>[2x]GS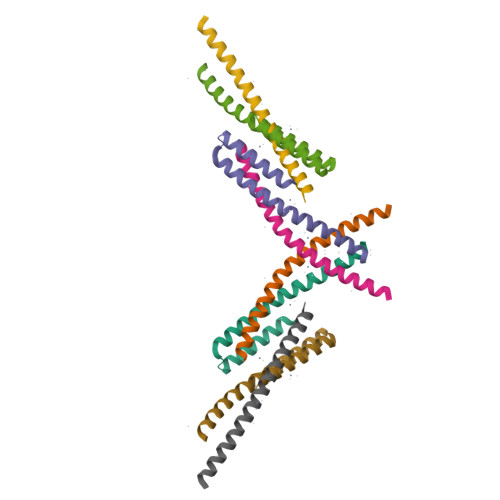SLENLPPVAASIEQLLERQWSEGQQFLLEQGTPSDILGMLKSLHQLQVENRRLEEQIKNLTAKKERLQLLNAQLS;>GTYEDLVQAQKEITAHNMQLREQTKQLEHDMAELRDQSQLLLKARCEELK[2x]> RHSRRA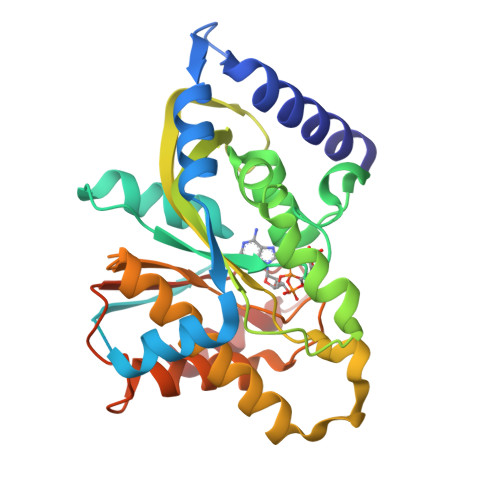IAAETVEILERGRYTAPSGRVVPIADHVAQAVRGTRLYRPEKLAVLLEGLGAASDGAPTRIEVTEETTLAAARRLTGAAGDQVACLNFASAEHPGGGFLSGAHAQEEGLARSSGLYASLRAVPQFYAFHHRQRDPLYSDHLIYSPGVPVFRDDAGRLLEEPYRVAFLTSPAPNRRAIGDLRTVEEIGRVLRGRAAKVLAAARHHGHRRLVLGAWGCGVFGNDPAQVAETFAGLLLDGGPFAGRFAHVVFAVWDTAPGAPRHAAFARRFGSL AcrIIA15 is an anti-CRISPR (Acr) protein that inhibits Staphylococcus aureus Cas9 (SaCas9). The AcrIIA15 protein, consisting of 170 amino acids, is comprised of two domains: an N-terminal domain (NTD) from residues 1 to 56, which contains a HTH motif resembling a transcriptional repressor, and a C-terminal domain (CTD) from residues 57 to 170. AcrIIA15, by combining the HTH domain and Cas9 inhibitory domain within a single protein, exhibits dual functionality as a bi-functional anti-CRISPR protein capable of both transcriptional repression and CRISPR-based cleavage inhibition. Our structural and biochemical studies demonstrate that AcrIIA15 functions as a dimer to simultaneously inhibit both anti-CRISPR operon transcription and SaCas9-sgRNA DNA recognition.

The HTH-containing NTD domain alone also binds to IRs with high affinity. To investigate how AcrIIA15 recognizes promoter DNA in a sequence-specific manner, we determined the crystal structures of the full-length AcrIIA15 or the NTD domain in complex with IR1 DNA at resolutions of 3.15 Å and 3.10 Å, respectively. AcrIIA15NTD consists of four α-helices, with helices α2 and α3 together forming the HTH motif. Specifically, helix α3 of the HTH domain inserts into the major groove of the DNA and forms three base contacts with two base-pairs in each IR sequence. Specifically, amino acids K31 and S25 form hydrogen bonds with the bases of the G6-C6′ pair. In addition, the sidechain of Q26 forms hydrogen bonds with the base of A4. Alanine substitutions at S25 and Q26 moderately reduced the binding affinity, and the single mutation K31A completely disrupted the interactions between the HTH and DNA. Importantly, these AcrIIA15 mutants fold properly, as confirmed by CD spectroscopy. These findings show that AcrIIA15NTD sequence-specifically recognizes the IR sequences through the establishment of base contacts between helix α3 and DNA. Specifically, amino acids S14, S15, N16, S30, and N34 establish interactions with the phosphate backbone of one DNA strand adjacent to the 5′-end. Additionally, residues K37, T43, and S46 interact with the phosphate groups of nucleotides in the middle spacing regions.

>SMRKTIERLLNSELSSNSIAVRTGVSQAVISKLRNGKKELGNLTLNSAEKLFEYQKEMEKVDT[4x]> ATTPTMQSTSLLTEHLGYPPISLVDDIINAVNEIMYKCTNAMEKYLMQRNIIGKKDFSDEIKIGTAKLESLLENSVDKNFDKLELYVLRNILSIPSDLLEENRFRLLHHEKLVLTDSATRAHTDTSIEQKLQEIERQYQLNVMLRDRIQNTKELLTEVVQFKKKVIDLLRCDDNLTTALHELWDDLKPLDVAVKLITTRLKQIYLENEEFYSIDQVNRLVKRYNELRNTSIVR;> MSVDRYSGMEGTEHIRFQRLVQVCNKALEESIRKLQSWEKIHECFPNYGQTREGIENLTVCQQQVIKLWSNLSRVEFDAIFHERSIEEKLNQLDDLINKARSIDTSSSSKKLRKIDDLRPLELIEGNLQGAKESTLERINNKLQIIKESNEALETNLKDLNDNIFQELDQLQQVYDDMLNEKSMLPDETIKQAVSDMIIESRQTS;> QLNDIISPHKDVHESEFYRYMNNSFAQDLKMKQLMNWCLIRAL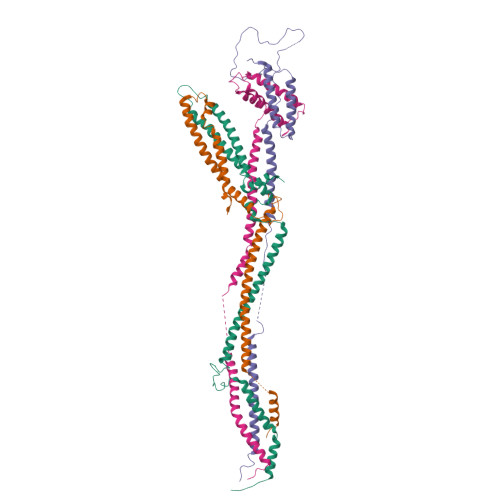RKLEIKNSQNKSESRKITLTILKDFVRDIRKGSHDIDWXXXXXXXXXXXXXXXXXXXXXXXXXXXXXXXXXXXXXXXXXXPPIKLAKIPNEKNIQNKENAKILEEKIKTIKNEIEQWSKDLSDVKIPSYELPKSQTSIVKLPDNLQLTATTKESIHSDFQKRVDGLQETTRLLKSSSILLNETAGMKLQRLNGCIVKKRPEDKNSTK;> MSSYVDKLDITQKQLRFLHKQFKEIIDEKVRTALPESSEDDQVSQEIQLQLDQFLMDVLEMAGESMNVVDAGKGTTVKSVIQEVQKEYTEPFDVELNEKVRKLYQEWEDETVKVSKLRREAPQVAVSEYTKQENQLLEEIDSLIAKMDSSQPNLQNEDQDEGQNEEKTQEYWNQVANQYGSILTSLKEINDKIPTHESKQKRLRLLLDLIEKEVAT>MGHHHHHHENLYFQGHFVQQKVKVFRAADPLVGVFLWGVAHSINELSQVPPPVMLLPDDFKASSKIKVNNHLFHRENLPSHFKFKEYCPQVFRNLRDRFGIDDQDYLVSLTRNPPSESEGSDGRFLISYDRTLVIKEVSSEDIADMHSNLSNYHQYIVKCHGNTLLPQFLGMYRVSVDNEDSYMLVMRNMFSHRLPVHRKYDLKGSLVSREASDKEKVKELPTL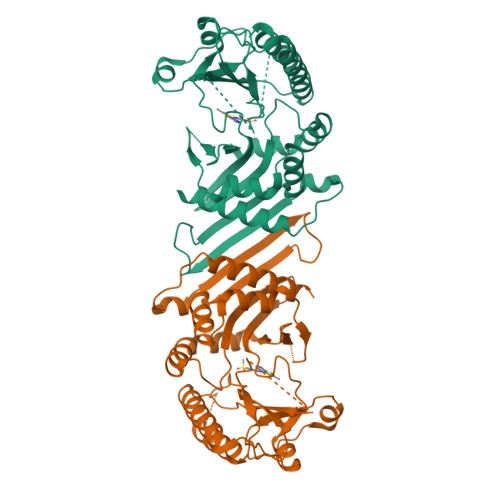KDMDFLNKNQKVYIGEEEKKIFLEKLKRDVEFLVQLKIMDYSLLLGIHDIIRGSEPEEELGPGEFESFIDVYAIRSAEGAPQKEVYFMGLIDILTQYDAKKKAAHAAKTVKHGAGAEISTVHPEQYAKRFLDFITNIFA[2x]>MSLMIKVEDMMTRHPHTLLRTHTLNDAKHLMEALDIRHVPIVDANKKLLGIVSQRDLLAAQESSLQRSAQGDSLAFETPLFEVMHTDVTSVAPQAGLKESAIYMQKHKIGCLPVVAKDVLVGIITDSDFVTIAINLLELQ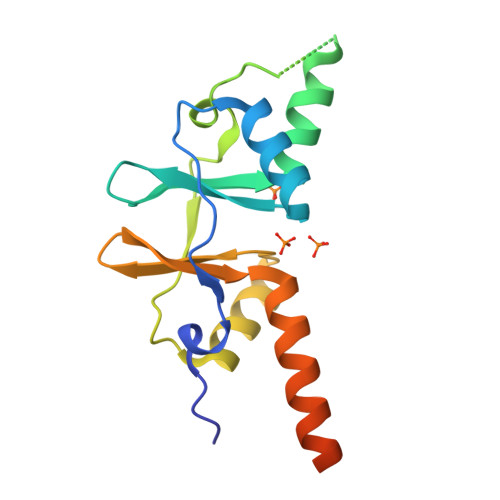EESEPDELDEEQEGHHHHHH[2x]>GEKKECWSWESYLEEQKAITAPVSLFQDSQAVTHNKNGFKLGMKLEGIDPQHPSMYFILTVAEVCGYRLRLHFDGYSECHDFWVNANSPDIHPAGWFEKTGHKLQPPKGYKEEEFSWSQYLRSTRAQAAPKHLFVSQSHSPPPLGFQVGMKLEAVDRMNPSLVCVASVTDVV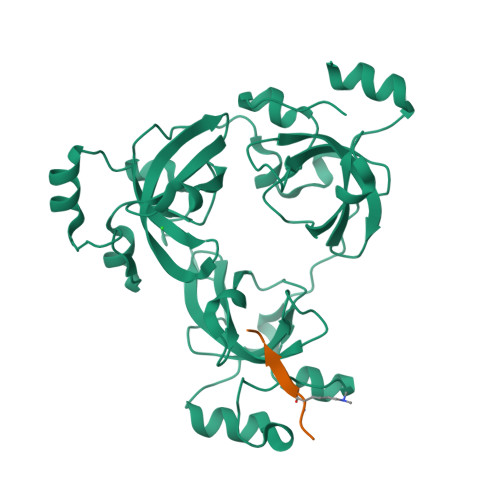DSRFLVHFDNWDDTYDYWCDPSSPYIHPVGWCQKQGKPLTPPQDYPDPDNFCWEKYLEETGASAVPTWAFKVRPPHSFLVNMKLEAVDRRNPALIRVASVEDVEDHRIKIHFDGWSHGYDFWIDADHPDIHPAGWCSKTGHPLQPPLGPREPSSASPGG[3x];>[2x]AKRHRKVLRDN Isovaleryl-CoA (coenzyme A) dehydrogenase (IVD) is an intramitochondrial flavoenzyme that catalyzes the conversion of isovaleryl-CoA (3-methylbutyryl-CoA) into 3-methylcrotonyl-CoA in the leucine catabolism pathway, transferring electrons to the electron-transferring flavoprotein (ETF). Consistent with other ACADs, including short-, medium-, and long-chain ACADs, IVD is characterized by a tetrameric architecture composed of 4 identical subunits. Each subunit of IVD contains one noncovalently attached FAD molecule, imparting a characteristic yellow color to the purified enzyme. Dysfunction of IVD is linked to isovaleric acidemia (IVA), a rare metabolic disorder characterized by the accumulation of toxic metabolites.

To elucidate the complex structure with its substrates, an IVD construct with the E286A mutation was expressed and purified for cryo-EM preparation to minimize conformational instability caused by the process of enzymatic reaction. Upon incubation with isovaleryl-CoA and butyryl-CoA, complexes of IVD with both substrates were resolved at resolutions of 3.35 and 2.91 Å, respectively. Following the addition of the 2 acyl-CoAs, the refinement process revealed additional tubular densities in the active site that ran partially parallel to the riboflavin portion of FAD, which were well-modeled as isovaleryl- and butyryl-CoA. FAD enters the pocket through a space formed at the junction of neighboring monomers, while the acyl-CoAs adhere to the surface of one monomer and enter through an opening on the opposite side, allowing their fatty acyl portions to interact with the FAD ring deep in the pocket. D284 and M280 form hydrogen bond interactions with adenosine at N6, while S222 and R223 contribute to interactions with the 3′-phosphate. These interactions confirm that the CoA on the outer part of the pocket is close to the monomer, while the remaining portion extends into the pocket, riveted by S174 and R287 from opposing directions. Although IVD can catalyze dehydrogenation of substrates ranging from C4 to C6, it exhibits the highest activity for isovaleryl-CoA, a C4 straight chain with a methyl group at the Cβ position. At the bottom of the active pocket, where the fatty acyl portion and the FAD ring reside, E286 extends its carboxyl group to approach the Cα–Cβ bond of the substrate to abstract proton. G406 and A407, located at a critical loop position in the middle of the helix, provide suitable space for the insertion of branched chains from substrates. Comparison of the 2 acyl-CoAs in terms of binding revealed a twist alternation at the fatty acyl portion, potentially attributed to the additional side-chain methyl constraining space within the pocket.

>[4x]MAEMATATRLLGWRVASWRLRPPLAGFVSQRAHSLLPVDDAINGLSEEQRQLRQTMAKFLQEHLAPKAQEIDRSNEFKNLREFWKQLGNLGVLGITAPVQYGGSGLGYLEHVLVMEEISRASGAVGLSYGAHSNLCINQLVRNGNEAQKEKYLPKLISGEYIGALAMSEPNAGSDVVSMKLKAEKKGNHYILNGNKFWITNGPDADVLIVYAKTDLAAVPASRGITAFIVEKGMPGFSTSKKLDKLGMRGSNTCELIFEDCKIPAANILGHENKGVYVLMSGLDLARLVLAGGPLGLMQAVLDHTIPYLHVREAFGQKIGHFQLMQGKMADMYTRLMACRQYVYNVAKACDEGHCTAKDCAGVILYSAECATQVALDGIQCFGGNGYINDFPMGRFLRDAKLYEIGAGTSEVRRLVIGRAFNADFH BISELENITE ION 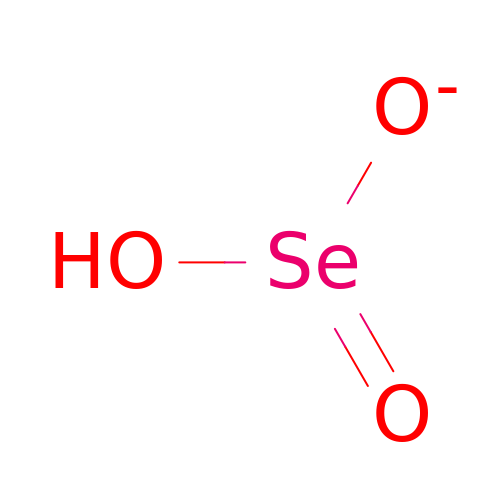| H O3 Se | MCAHWIHFGHIESP-UHFFFAOYSA-M> SMEQPEPDMITIFIGTWNMGNAPPPKKITSWFLSKGQGKTRDDSADYIPHDIYVIGTQEDPLSEKEWLEILKHSLQEITSVTFKTVAIHTLWNIRIVVLAKPEHENRISHICTDNVKTGIANTLGNKGAVGVSFMFNGTSLGFVNSHLTSGSEKKLRRNQNYMNILRFLALGDKKLSPFNITHRFTHLFWFGDLNYRVDLPTWEAETIIQKIKQQQYADLLSHDQLLTERREQKVFLHFEEEEITFAPTYRFERLTRDKYAYTKQKATGMKYNLPSWCDRV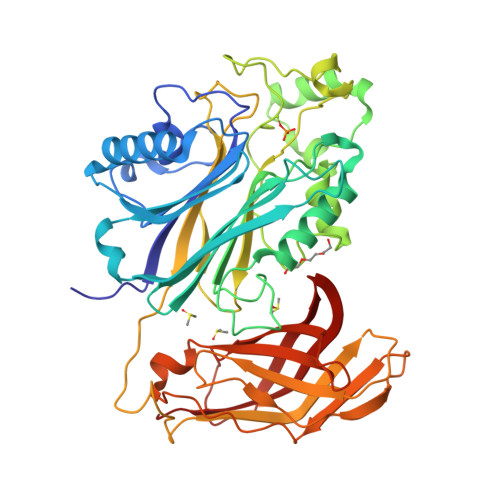LWKSYPLVHVVCQSYGSTSDIMTSDHSPVFATFEAGVTSQFVSKNGPGTVDSQGQIEFLRCYATLKTKSQTKFYLEFHSSCLESFVKSQEGENEEGSEGELVVKFGETLPKLKPIISDPEYLLDQHILISIKSSDSDESYGEGCIALRLEATETQLPIYTPLTHHGELTGHFQGEIKLQTSQ>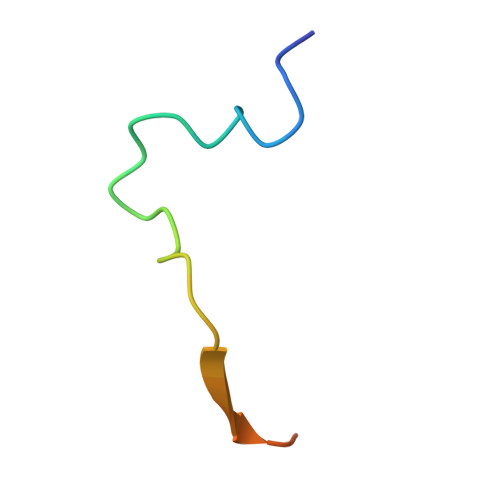 APKFGDWDENNPSSADGYTHIFNKVRDEVD> TLSSQDKPFNLRSRDPIYSNNYGKLYEITPEKNSQLRDLDILLNCLQMNEGALFVPHYNSRATVILVANEGRAEVELVGLEQQQQQGLESMQLRRYAATLSEGDIIVIPSSFPVALKAASDLNMVGIGVNAENNERNFLAGHKENVIRQIPRQVSDLTFPGSGEEVEELLENQKESYFV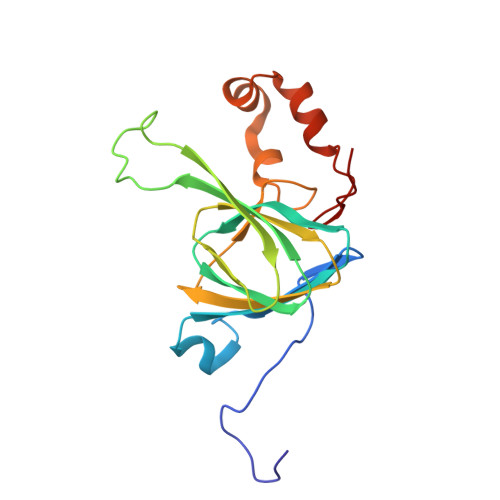DGQPR> MSNLLGPRDANGIPVPMTVDESIASMKASLLKKIKRSAYVYRVDCGGCNGCEIEIFATLSPLFDAERFGIKVVPSPRHADILLFTGAVTRAMRSPALRAWQSAPDPKICISYGACGNSGGIFHDLYCVWGGTDKIVPVDVYIPGCPPTPAATLYGFAMALGLLEQKIHARGPGELDEQPAEILHGDMVQPLRVKVDREARRLAGYRYGRQIADDYLTQLGQGEEQVARWLEAENDPRLNEIVSHLNHVV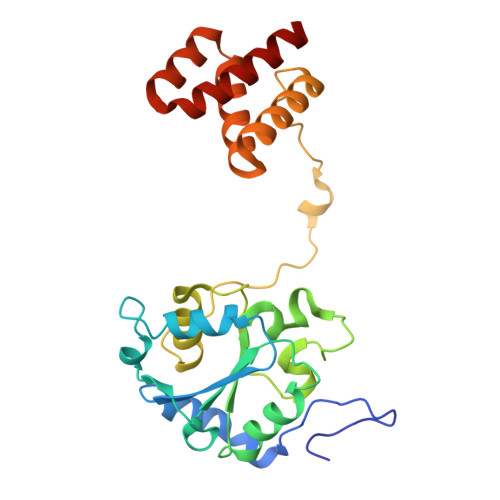EEARIR>ADVFHLGLTKAMLDGATLAIVPGDPERVKRIAELMDNATFLASHREYTSYLAYADGKPVVICSTGIGGPSTSIAVEELAQLGVNTFLRVGATGAIQPHVNVGDVIVTQASVRLDGASLHFAPMEFPAVANFECTTAMVAACRDAGVEPHIGVTASSDTFYPGQERYDTVT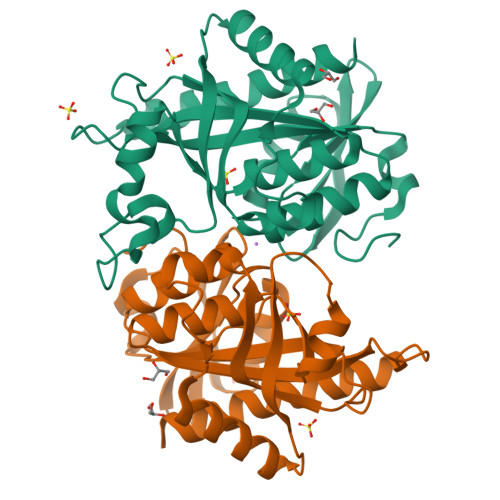GRVTRRFAGSMKEWQDMGVLNYEMESATLFTMCATQGWRAACVAGVIVNRTQQEIPDEATMKKTEVSAVSIVVAAAKKLLA[2x]>MNYTILKFKTIN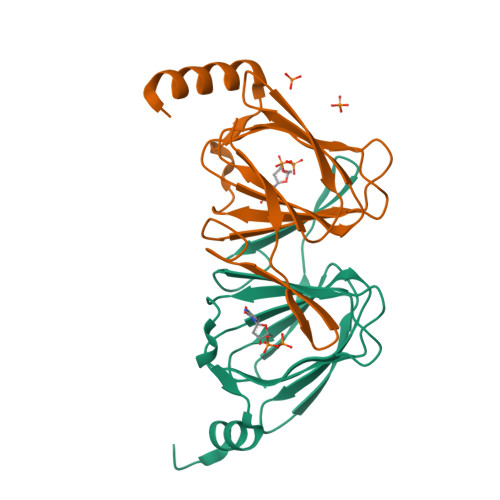SKNSILNVHQKDVNCPFEIKRIFYIYDFLDDSIRGDHANLNSEFIFIALNGSCEILIDDGKTKQKIILNNKTKGLYIDKMIWKQMYNFSKDCILLVLTNTYYDEKEYIYDYKYFCELKNNIVWRGGYAIKTMPLEHHHHHH[3x]>[2x]GVLKGINFDRSIVTPENEASILDLAMQNRSGVLDGMTIDILNTTSNQLALFHGTAVLQG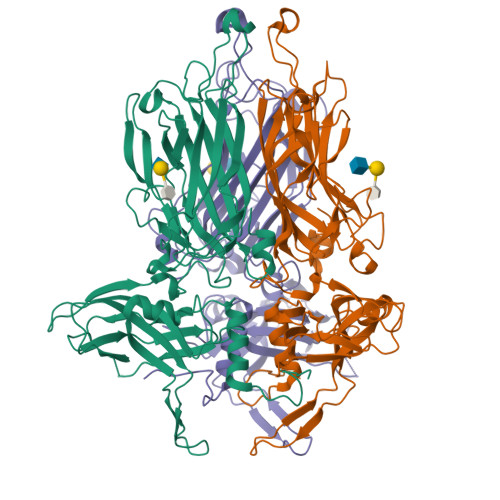YGIEITRAANGAPDVLVDTTGQSNETMLLCLTIDLNQVNVPSGTVGTNTYAVDYKQIRLEFLDVPTLLKQYWRDHSLHDLIDPRRVISMPLYWITFGQTGTTPKYEQIKSNYIDGGNSGNPAYGIAARCENFNHFINKVAVQSIPINGVANRPVSSTASQLTNYKVWRNPYLCSQDPRDKFAPDNLVIEEDGIYRIDISGSINIANYTFPASGNSWRVGGRYFQIVCARNSSANNLAEFGAEQHLPPSGVWTRRVLVGEYTAGMTEQAFSSVATISLFKGDNFFLQFETGTNTSRDSAYNNGYGTSGTHLRNFSYTLERVGDLNGTAYYDNGTF> MNFEWTHEQAELFEHALRFGKELSAPLQEDNGFPRDNWNALGDFGYFGLPIPEKYAKDGSGFDILTTIKIIEGLGQSCTDTGLLFAGAAHTFACSMPILEHGSETLKHQLLPDLATGRKIAANAISEASAGSDISNLATTAQKEGD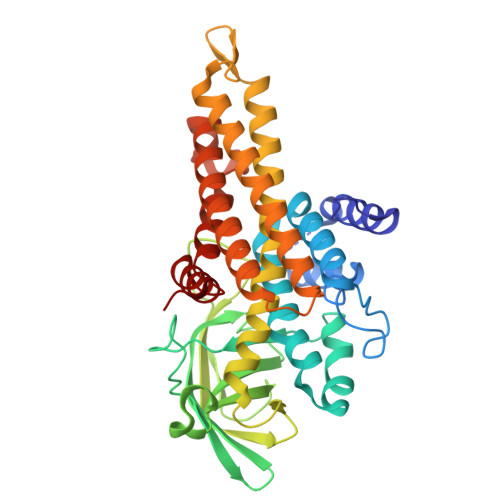YYVLNGGKSYVTNGSIADYYVVYATTNKKHGYLGQTAFVVPRNTPGISVGNDYHKLGLRSAPLNQVFFDNCTIHKDYALGREGQGARIFAASMDWERCCLFAIFVGAMQRDLNQCIEYANTRMQGDKTISRFQAVSHRIADMGVRLESARLMLYYAAWQKSQDVDNTKAVAMSKLAISEAFVQSGIDSIRVHGALGYLDEGRVNNSIKDALGSVLFSGTSDIQRELICNRLGLL> PTSKPTTTGKGCHIGRFKSLSPQELASFKKARDALEESLKLKNWSCSSPVFPGNWDLRLLQVRERPVALEAELALTLKVLEAAAGPALEDVLDQPLHTLHHILSQLQACIQPQPTAGPRPRGRLHHWLHR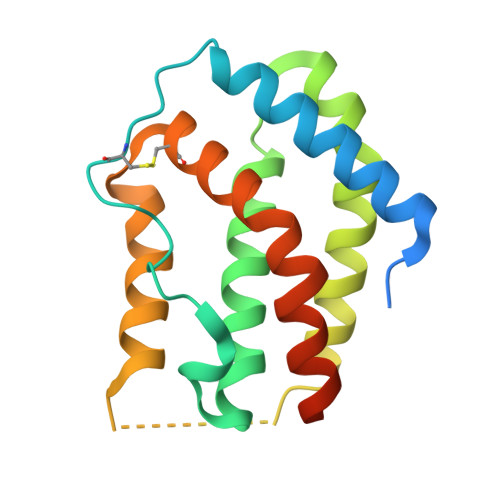LQEAPKKESAGCLEASVTFNLFRLLTRDLKYVADGNLCLRTSTHPEST>[4x]SAVKTNVGPSRAGVGYDVIVIGGGFAGVTAAREASRSGLKTLILEGRSRLGGRTFTSKLQNQKVELGGTWVHWTQPNVWTEIMHYGLEVEETVGLANPETVIWVTEDNVKRAPAAEAFEIFGSACNEYYKEARNIYPRPFEPFFERKKLQHVDGLSAADYLEKLPLTREQKDMMDSWLSGNGHNYPETIAYSEIMRWFALSNFNMPTMFDSIARYKIKTGTHSLLEAIMADGNSEVKLSTPVTKVNQDKDKVTVTTEDGVFTASAVIVAVPINTLHDIEYSPKLSAAKVDMGSQRHAGAGVKGYIRVKQNVGNVMTYAPARNKLTPFTSVFTDHVDESGTLLIAFSADPKLIDINDIKAVEKALQPLLPGVEVTASYGYDWNLDPFSKGTWCTYRPNQTTRYLTELQKREGRLFFAGSDMANGWRGFIDGAIENGREVGHQVATYLKRENDNA

The first two steps in the pathway are catalyzed by the enzymes nicotine oxidoreductase (NicA2) and pseudooxynicotine amine oxidase (Pnao), which convert nicotine into pseudooxynicotine (Pon) and Pon into 3-succinoylsemialdehyde-pyridine, respectively. Both NicA2 and Pnao are members of the widespread flavin-dependent amine oxidase enzyme family. Enzymes of this family use a flavin adenine dinucleotide (FAD) prosthetic group to accept a hydride from their amine containing substrate, forming an oxidized product and reduced flavin hydroquinone (FADH2) in the reductive half reaction. However, our lab recently demonstrated that NicA2 is instead a dehydrogenase that uses a cytochrome c protein (called CycN) as a biological oxidant.

The crystal structure of Pnao was solved at 2.60 Å resolution. The structure of the Pnao monomer has a similar overall architecture as NicA2 (39% identity, RMSD of 1.5 Å), firmly placing Pnao in the flavoprotein amine oxidase enzyme family. The asymmetric unit indicated that Pnao exists as a homodimer with a similar dimer interface as NicA2. Overlaying the Pnao structure with the nicotine-bound structure of NicA2 reveals that the substrate binding pocket in Pnao is considerably deeper than that in NicA2 due to a replacement of Trp364 in NicA2 with Ser372 in Pnao. Trp364 forms the backstop of NicA2’s substrate binding site and forms hydrophobic interactions with the pyridine ring of nicotine; replacing it with Ser372 in Pnao allows for a more extended substrate binding cavity that is presumably better able to accommodate the more extended Pon substrate relative to nicotine. In Pnao, the aromatic cage residues are Trp434 and Phe470, which are more typical residues that compose the aromatic cage in this enzyme family. Several of the aromatic residues in the substrate binding site of NicA2 (Trp108, Tyr214, and Trp434) are the same or similar in Pnao (Trp113, Trp220, and Trp434) and may promote the hydrophobicity of the “aromatic cage” commonly found in flavoprotein amine oxidases. Ser372 is appropriate positioned to form a hydrogen bond with the pyridine nitrogen of Pon, and the deeper substrate binding pocket due to the presence of Ser372 may allow aromatic stacking of Trp220 with the pyridine ring of Pon in Pnao. However, the isoalloxazine is buried in both NicA2 and Pnao, with the C7–C8 edge of the isoalloxazine >10 Å away from the protein surface in both enzymes. Our structure of Pnao contained oxidized FAD, and it therefore remains possible that a change in conformation occurs upon reduction to the semiquinone that occludes the isoalloxazine from the solvent and reduction by dithionite.1H-imidazol-5-ylmethanol | C4 H6 N2 O 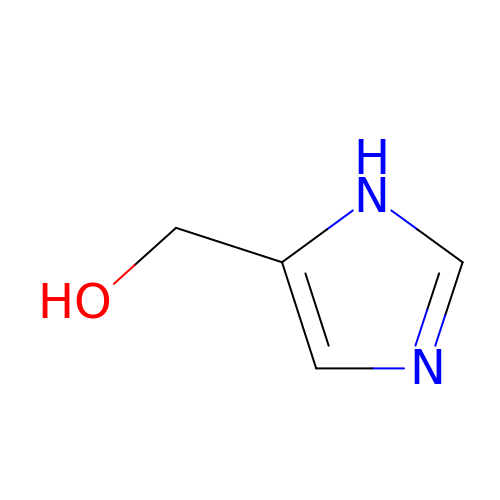| QDYTUZCWBJRHKK-UHFFFAOYSA-N>[6x]GSHMASMTGGQQMGRGSMSKIVKIIGREIIDSRGNPTVEAEVHLEGGFVGMAAAPSGASTGSREALELRDGDKSRFLGKGVTKAVAAVNGPIAQALIGKDAKDQAGIDKIMIDLDGTENKSKFGANAILAVSLANAKAAAAAKGMPLYEHIAELNGTPGKYSMPVPMMNIINGGEHADNNVDIQEFMIQPVGAKTVKEAIRMGSEVFHHLAKVLKAKGMNTAVGD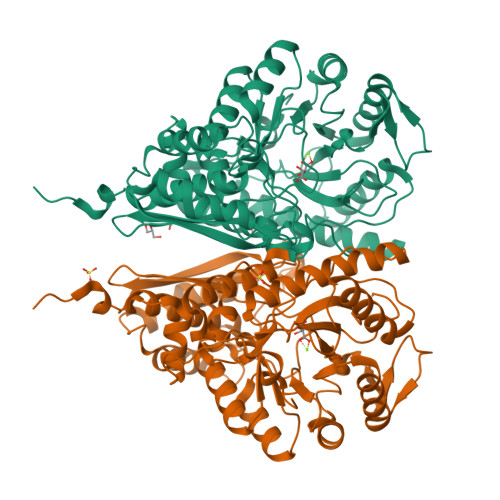EGGYAPNLGSNAEALAVIAEAVKAAGYELGKDITLAMDCAASEFYKDGKYVLAGEGNKAFTSEEFTHFLEELTKQYPIVSIEDGLDESDWDGFAYQTKVLGDKIQLVGDDLFVTNTKILKEGIEKGIANSILIKFNQIGSLTETLAAIKMAKDAGYTAVISHRSGETEDATIADLAVGTAAGQIKTGSMSRSDRVAKYNQLIRIEEALGEKAPYNGRKEIKGQA>[4x]MKKIYLIRHAQSEYNEKGIFQGRLDSDLTPLGFVQSRLLVKQFEREKPEVIITSPQRRAYKTALTLSDVLGIDLIVDERIREMSFGVLEGRHFWTMFEENKEMIINWLKDPVKYPLPTQEDIKEFEKRIKEFLEDLKSRKEKVLAVVGHGGTLHGLLCLALGIGLEKMWHIHMDNTGISLLEYDGERFYLKSLNDTCHLLVLD

The riboflavin biosynthetic pathway is well-studied with dedicated enzymes to perform complex chemical transformations, with the exception of an unknown phosphatase that catalyzes the dephosphorylation of ARAPDP, the product of RibD, to generate 5-amino-6-ribitylamino-pyrimidinedione (ARAPD), the substrate for lumazine synthase. Using an anaerobic activity-based screen, two phosphatases from Aquifex aeolicus were identified that dephosphorylate ARAPDP, but only one reconstitutes riboflavin production in a one-pot experiment with the other four enzymes of riboflavin biosynthesis. The structures of both enzymes were determined by X-ray crystallography to reveal the vastly different folds capable of performing the ARAPDP dephosphorylation chemistry.

The second enzyme, a histidine family phosphatase, only dephosphorylates ARAPDP in the one-pot experiment thus facilitating riboflavin formation. The structure of HFP was determined to 2.04 Å by single anomalous dispersion using selenomethionine substituted protein. HFP, like all histidine family phosphatases, is composed of α/β/α sandwich where the central six stranded β-sheet has one antiparallel strand. HFP is a dimer in solution, as estimated by preparative gel filtration chromatography. The HFP active site, or “phosphate pocket,” contains four highly conserved residues characteristic of all histidine family phosphatases, R8, H9, R58, and H149, as determined by sequence and structure alignments. Based on published mechanisms for homologous phosphatases, it is logical to propose that residues R8, R58, and H149 form hydrogen bonds and electrostatic interactions with the bound phosphate group of the substrate, while H9 accepts the phosphate from the substrate, assisted by a proton donor, likely E82. Water hydrolysis of the phospho-H9 is assisted by the proton donor, E82, resetting the active site for further turnover. There is significant density in the phosphate site that was modeled as sulfate derived from the crystallization conditions. Phe93, Trp107, and Trp169 form a hydrophobic the cavity that would enclose the pyrimidinedione of ARAPDP, similar to hydrophobic pocket generated by Val11, Val15, and Trp181 in RosC. The HFP identified in this study has the appropriate specificity against substrates of riboflavin biosynthesis to be a dedicated phosphatase for this pathway.>[2x]GPHMASALVMKKGQRLSRDALRTQLDSAGYRHVDQVMEHGEYATRGALLDLFPMGSELPYRLDFFDDEIDSLRVFDVDSQRTLEEVEAINLLP;>GPHMASTVSQMVDNVLSQPEGKR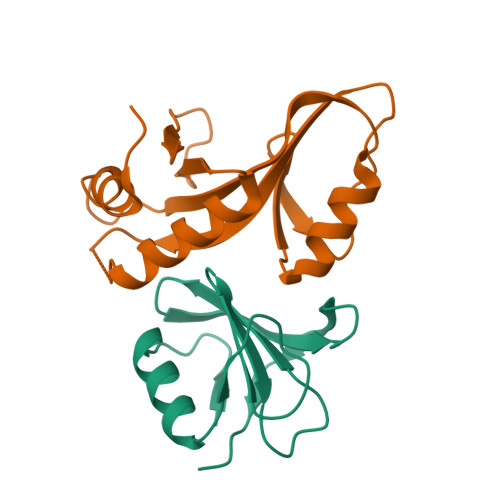LMLLAPIIKERKGEHTKTLENLASQGYIRARIDGEVCDLSDPPKLELQKKHTIEVVVDRFKVRDDLTQRLAESFETALELSGGTAVVADMDDPKAEELLFSAN[2x]> MAQYYPGTSKVAQNRRNFCNPEYELEKLREISDEDVVKILGHRAPGEEYPS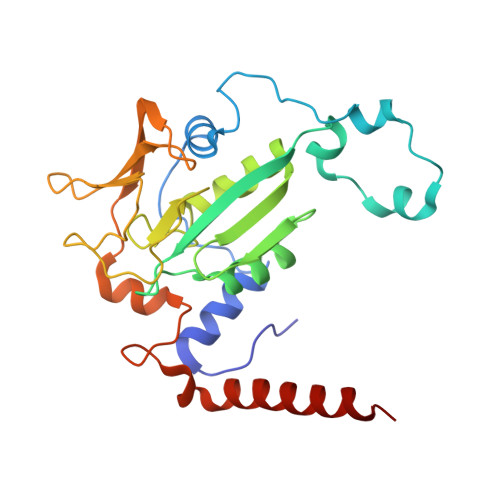VHPPLEEMDEPEDAIREMVEPIDGAKAGDRVRYIQFTDSMYFAPAQPYVRSRAYLCRYRGADAGTLSGRQIIETRERDLEKVSKELLETEFFDPARSGVRGKSVHGHSLRLDEDGMMFDMLRRQIYNKDTGKVEMVKNQIGDELDEPVDLGEPLDEETLMDKTTIYRVDGEAYRDDVEAVEIMQRIHVLRSQGGYNPE> MGSRSSHAAVIPDGDSIRRETGFSQASLLRLHHRFRALDRNKKGYLSRMDLQQIGALAVNPLGDRIIESFFPDGSQRVDFPGFVRVLAHFRPVEDEDTETQDPKKPEPLNSRRNKLHYAFQLYDLDRDGKISRHEMLQVLRLMVGVQVTEEQLENIADRTVQEADEDGDGAVSFVEFTKS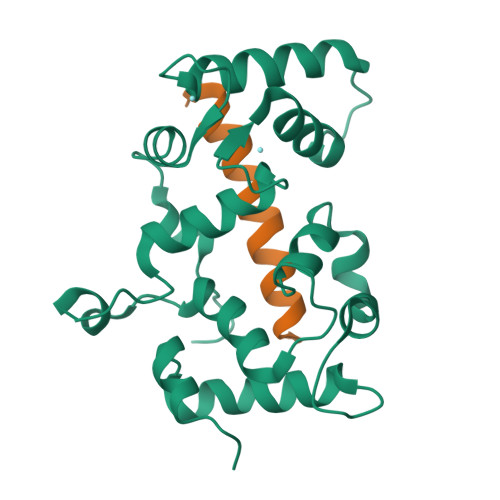LEKMDVEQKMSIRILKHHHHHH;> VDLLAVKKKQETKRSINEEIHTQFLDHLLTGIEDICGHYGHHH>[2x]MTEPDTERKGSSRRGFLAGLGAAALTGAGIGMAAGEVLRPLLPDSDPAASPKAEQRLRMAAQRADATAAPQPGISGPAPAFVHVIALDLAEEARKNPDTARDSAA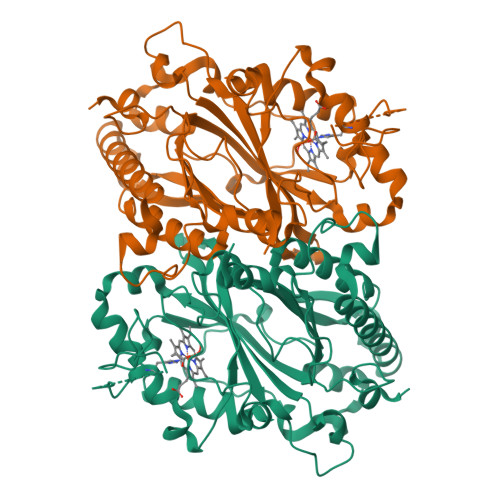AALRSWTELAARLHEESPHDIAEGAASAGLLPASLMVTVGIGGSLLSAIDAEDRRPDALADLPEFSTDDLHPRWCGGDFMLQVGAEDPMVLTAAVEELVAAAADATAVRWSLRGFRRTAAAARDPDATPRNLMGQIDGTANPAQDHPLFDRTITARPADNPAHAWMDGGSYLVVRRIRMLLTEWRKLDVAARERVIGRRLDTGAPLGSRNETDPVVLSARDEEGEPLIPENAHVRLASPENNLGARMFRRGYSYDQGWRDDGVRDAGLLFMAWQGDPATGFIPVQRSLADQGDALNRYIRHEGSALFAVPAAREGRYLGQDLIEG>[2x]MSVEKIPGYTYGETENRAPFNLEDLKLLKEAVMFTAEDEEYIQKAGEVLEDQVEEILDTAYGFVGSHPHL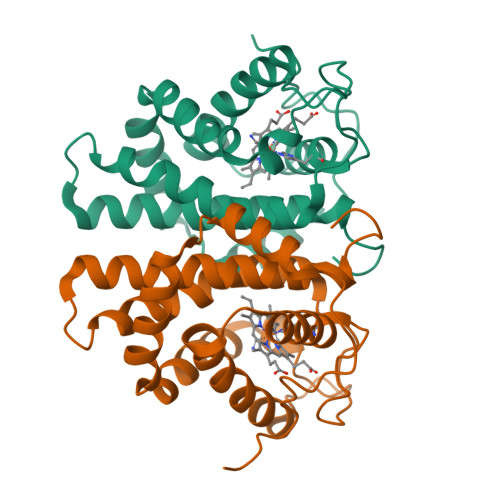LYYFTSPDGTPNEKYLAAVRKRFSRWILDTSNRSYDQAWLDYQYEIGLRHHRTKKNQTDNVESVPNIGYRYLVAFIYPITATMKPFLARKGHTPEEVEKMYQAWFKATTLQVALWSYPYVKYGDF>MGPMPKLADRKLCADQECSHPISMAVALQDYMAPDCRFLTIHRGQVVYVFSKLKGRGRLFWGGSVQGDYYGDLAARLGYFPSSIVREDQTLKPGKVDVKTDKWDFYCQ[2x]

Melanoma inhibitory activity (MIA), an extracellular 11 kDa protein highly expressed and secreted by melanoma cells after their malignant transformation, is known to play a key role in melanoma development, progression, and tumour cell invasion. Structural analysis revealed that MIA is a single domain protein that adopts an Src Homology 3 (SH3) domain-like fold with N- and C-terminal extensions. However, unlike classical SH3 domains, MIA does not bind proline-rich peptide ligands. After its secretion, MIA directly interacts with extracellular matrix molecules, such as laminin, fibronectin, and tenascin; it thereby masks the binding site of cell adhesion receptors, e.g. integrin, to these extracellular matrix components.

To elucidate the binding mode of all confirmed fragment hits, we soaked crystals of apo MIA with the individual fragments and determined the resulting structures by X-ray crystallography. As fragment soaking always led to a loss of crystal order, structural elucidation was only possible for protein crystals cross-linked with glutaraldehyde. Only for fragment 11 (pyrimidin-2-amine) we were able to obtain a complex with MIA in the protein crystals. The structure of fragment 11 bound to MIA was solved at a resolution of 1.39 Å in a primitive orthorhombic space group (P212121). The electron density unambiguously identifies the binding mode of fragment 11 that sits deeply within the hydrophobic cavity formed by L76, G77, and Y78. The binding involves a sandwich arrangement of the ring system of Y78 and the side chain of L76, consistent with the high- and low-field shift pattern of ligand induced chemical shift perturbations observed in 2D 1H-15N HSQC NMR spectra of MIA. The pyrimidine ring is stabilized by the hydrophobic residues L76, G77, and Y78 at the deepest part of the binding cleft. In addition to these hydrophobic packing interactions, the polar amino group of fragment 11 is orientated to C-terminal residues of MIA and forms a specific hydrogen bond with the backbone carbonyl oxygen of W102. Moreover, the pyrimidine nitrogen atoms N1 and N2 are involved in water-mediated hydrogen bonds with both the side chain of D103 and the main chain of R36, respectively. As such, fragment 11 occupies the position of a water molecule in the ligand-free structure that is displaced upon binding.> SEFENPLKRLLVPGEEWEFEVTAFYRGRQVFQQTISCPEGLRLVGSEVGDRTLPGWPVTLPDPGMSLTDRGVMSYVRHVLSCLGGGLALWRAGQWLWAQRLGHCHTYWAVSEELLPNSGHGPDGEVPKDKEGGVFDLGPFIVDLITFTEGSGRSP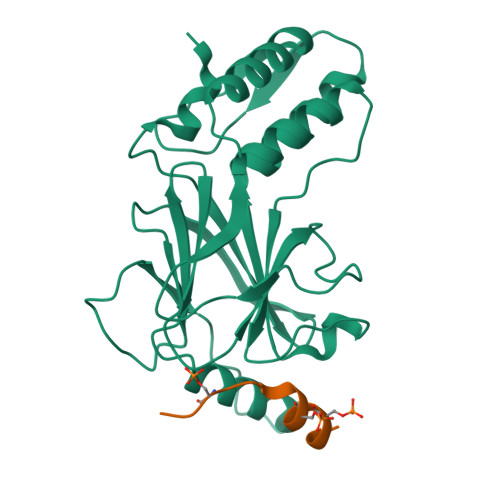RYALWFCVGESWPQDQPWTKRLVMVKVVPTCLRALVEMARVGGASSLENTVDLHISNSHPLSLTSDQYKAYLQDLVEGMDFQGPGES;> SPASLASNLEISQSPTMPFWS> SMAATAAEAVASGSGEPREEAGALGPAWDESQLRSYSFPTRPIPRLSQSDPRAEELIENEEPVVLTDTNLVYPALKWDLEYLQENIGNGDFSVYSASTHKFLYYDEKKMANFQNFKPRSNREEMKFHEF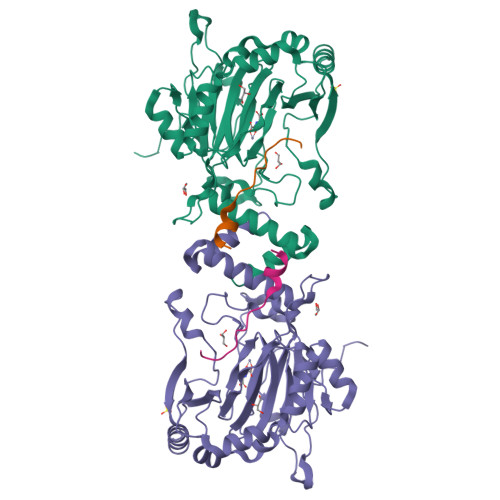VEKLQDIQQRGGEERLYLQQTLNDTVGRKIVMDFLGFNWNWINKQQGKRGWGQLTSNLLLIGMEGNVTPAHYDEQQNFFAQIKGYKRCILFPPDQFECLYPYPVHHPCDRQSQVDFDNPDYERFPNFQNVVGYETVVGPGDVLYIPMYWWHHIESLLNGGITITVNFWYKGAPTPKRIEYPLKAHQKVAIMRNIEKMLGEALGNPQEVGPLLNTMIKGRYN;> LHRASLFDHHELADYLISVGADINKID>GPGSMSDYETLRIRRDGYVLVIGLNRPAKRNAFDKTMLEELALALGEYETDTDLRAAVLYGEGPLFTAGLDLASVAAEIQGGASLTPEGGINPWQVDGRQLSKPLLVAVHGKVLTLGIELALAADIVIADETATFAQLEVNRGIYPFGGATIRFPRTAGWGNAMRWMLTADTFDAVEAHRIG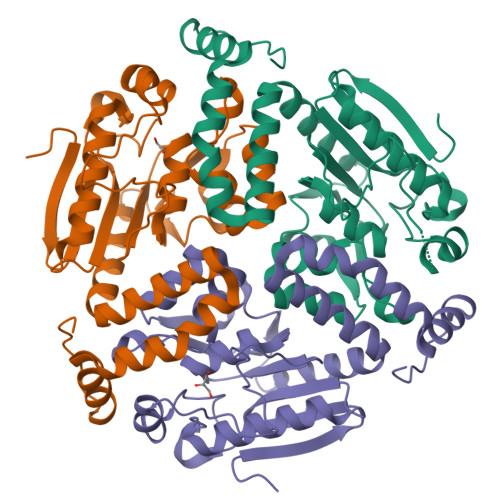IVQEIVPVGEHVDTAIAIAQTIARQAPLGVQATLRNARLAVREGDAAAEEQLVPTVRELFTSEDATLGVQAFLSRTTAEFVGR[3x]> QSHDEIIDKLIERTNKITTSISHVESLLDDRLDPKRIRKAGSLRHRVEELEDPSCDEHEHQCGGDDPQCISKLFVCDGHNDCRNGED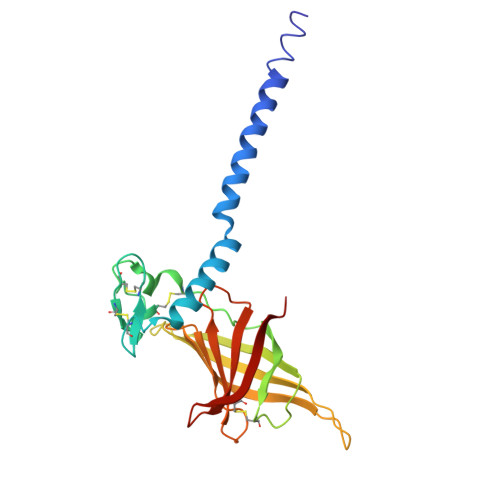EKDCTLPTKAGDKFIGDVCFDHCTKRRPEHMTLAFESSSIAAFFTPIADLHVHIEIESETDEDESEVSMPADGEYSFADHRLTIHPPEEDGLGLVGEFDGYNFDRFVGHIVHELSEEVCAEFIFHRKK> MHHHHHHHHHHSGQNLYFQGHMATFISVQLKKTSEVDLAKPLVKFIQQTYPSGGEEQAQYCRAAEELSKLRRAAVGRPLDKHEGALETLLRYYDQICSIEPKFPFSENQICLTFTWKDAFDKGSLFGGSVKLALASLGYEKSCVLFNCAALASQIAAEQNLDNDEGLKIAAKHYQFASGAFLHIKETVLSALSREPTVDISPDTVGTLSLIMLAQAQEVFFLKATRDKMK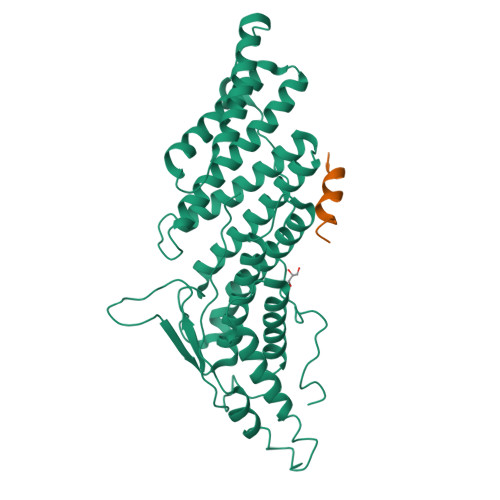DAIIAKLANQAADYFGDAFKQCQYKDTLPKEVFPVLAAKHCIMQANAEYHQSILAKQQKKFGEEIARLQHAAELIKTVASRYDEYVNVKDFSDKINRALAAAKKDNDFIYHDRVPDLKDLDPIGKATLVKSTPVNVPISQKFTDLFEKMV;> DEEALKQLAEWVS>[6x]SPPAVPQTFQVAHLHAPTGSGKSTKVPAAYAAQGYKVLVLNPSVAATLGFGAYMSKAH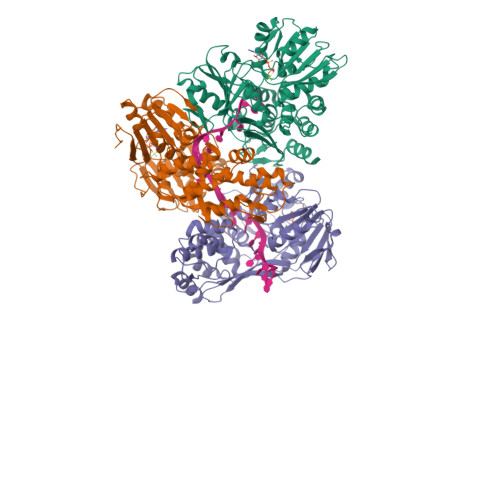GIDPNIRTGVRTITTGAPITYSTYGKFLADGGCSGGAYDIIICDECHSTDSTTILGIGTVLDQAETAGARLVVLATATPPGSVTVPHPNIEEVALSSTGEIPFYGKAIPIETIKGGRHLIFCHSKKKCDELAAKLSGLGLNAVAYYRGLDVSVIPTSGDVIVVATDALMTGFTGDFDSVIDCNTCVTQTVDFSLDPTFTIETTTVPQDAVSRSQRRGRTGRGRMGIYRFVTPGERPSGMFDSSVLCECYDAGCAWYELTPAETSVRLRAYLNTPGLPVCQDHLEFWESVFTGLTHIDAHFLSQTKQAGDNFPYLVAYQATVCARAQAPPPSWDQMWKCLIRLKPTLHGPTPLLYRLGAVQNEVTTTHPITKYIMACMSA>[2x]GPKSSDHVDLPYNLTATKIDSDVFVVTDRDFCSSNVLVAKMLDGTVVIVSSPFENL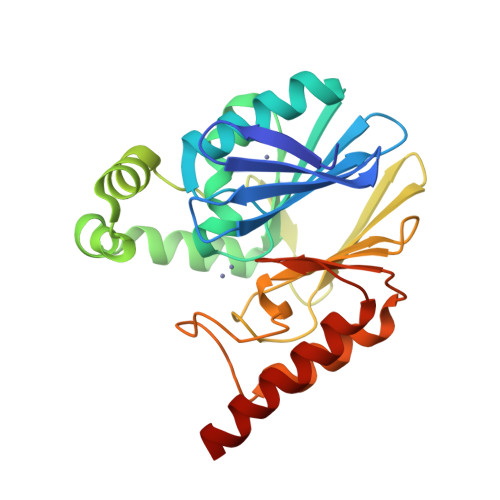GTQTLMDWVAKTMKPKKVVAINTHFHLDGTGGNEIYKKMGAETWSSDLTKQLRLEENKKDRIKAAEFYKNEDLKRRILSSHPVPADNVFDLKQGKVFSFSNELVEVSFPGPAHSPDNVVVYFPKKKLLFGGCMIKPKELGYLGDANVKAWPDSARRLKKFDAKIVIPGHGEWGGPEMVNKTIKVAEKAVGEMRL2'-DEOXY-5-NITROURIDINE 5'-MONOPHOSPHATE | C9 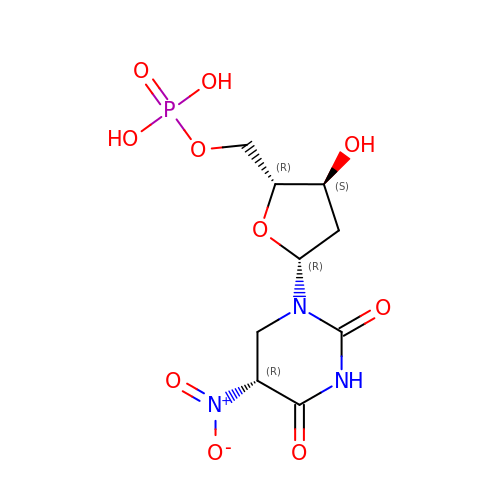H14 N3 O10 P | ZYBJIJYGXJSDTC-XZBKPIIZSA-N>[4x]MRGSHHHHHHGSSAVSTTAAPEARSILAGAAEGKVIATTEALSFWGGVDPATGKVIDVHHPLHGICLTGGVLFMPTSRGACTGSGVLLDLILTGRAPSALVFCEAEDVLTLGALVAAEMFDKALPVIRLDTETFARFSRAAHVRIDQNTIKADGVSLAVAPPATAHLDLTDDDRAMLEGRDGIAVRQAMRIIVAMAAQQGASALVDVTQGHIDGCIYASPANLTFAEKMADMGGKVRVPSTMNAISVDKANWRAQGVPEDFGDPAARLADAYVRMGCRPTFTCSPYLLDSAPSAGESIGWAESNAVIFANTVLGARTAKHPDFLDLCIAMTGRAPLSGVYLEENRRPQRIVDVALPAGIDDAFWPLVGYLAGKAVPDCIPLLRGLGAAKPSRDDLKALCAAFGTTSASPMLHIEGATPEAGLAPLETAETVTISLEDMAAGWSLLNEGPEEVQLVAIGSPHASLEECRALAAVFNGRKRHADVAVIVTAGQQVIDAAGKDGTLQ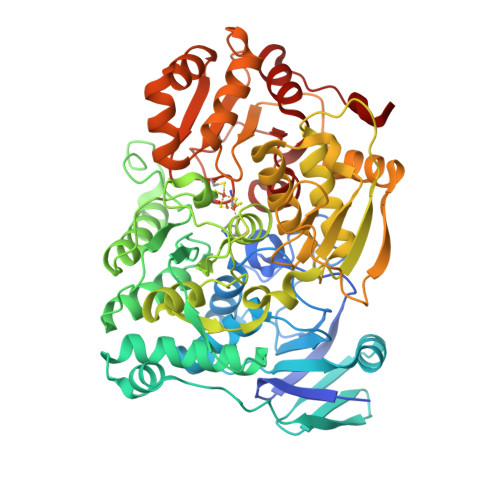SLKDSGVQVLPDLCWCSISEPVFPTKTRALMTNSGKYAHYGPGLSGRAVRFGSLADCVESALTGRAVSRLPVWLS(1R,5aS,6R)-1,2,5,5a,6,7-hexahydrophenazine-1,6-dicarboxylic 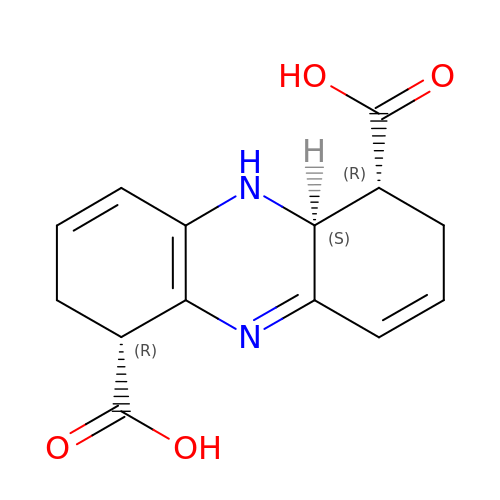acid | C14 H14 N2 O4 | FXTPBWZKMDQSSJ-XLDPMVHQSA-N>GIPKCPEDWGASSRTSLCFKLYAKGKHEKKTWFESRDFCRALGGDLASINNKEEQQTIWRLITASGSYHKLFWLGLTYGSPSEGFTWSDGSPVSYENWAYGEPNNYQNVEY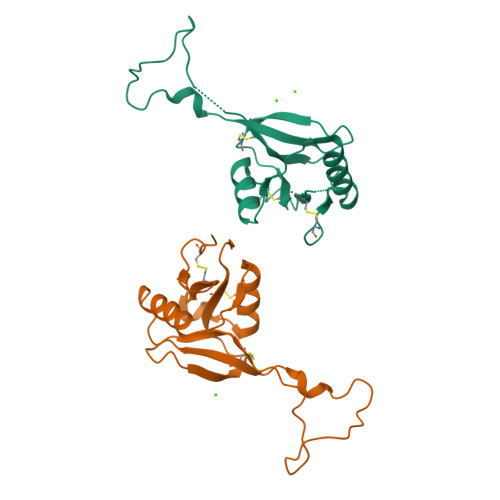CGELKGDPTMSWNDINCEHLNNWICQIQKGQTPKPD[2x]>[2x]ALPDLKIEKLEEGVFVHTSFEEVNGWGVVTKHGLVVL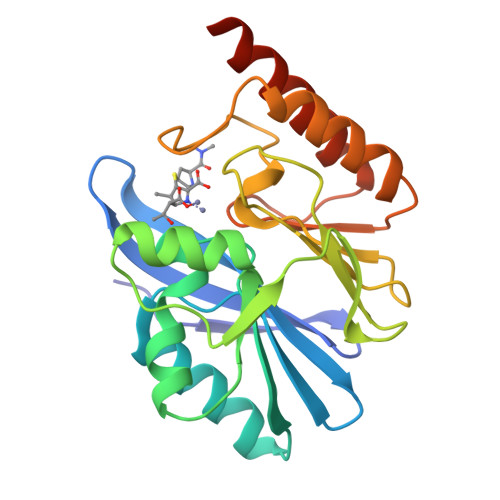VNTDAYLIDTPFTATDTEKLVNWFVERGYEIKGTISSHFHSDSTGGIEWLNSQSIPTYASELTNELLKKSGKVQAKYSFSEVSYWLVKNKIEVFYPGPGHTQDNLVVWLPESKILFGGCFIKPHGLGNLGDANLEAWPKSAKILMSKYGKAKLVVSSHSEKGDASLMKRTWEQALKGLKESKKTSSPSN3,6-dideoxy-L-arabino-hexonic acid | C6 H12 O5 | 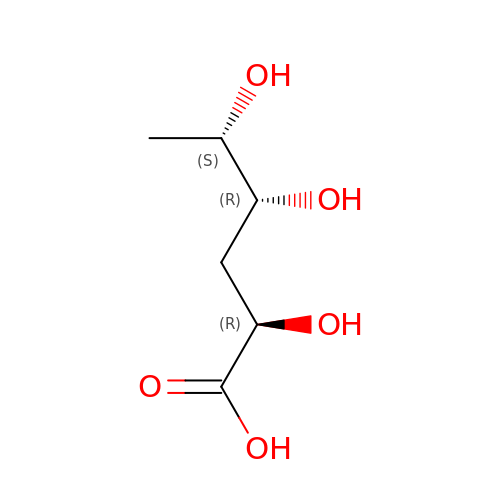RJZYGPZBSUBNEJ-VPENINKCSA-N The arsN1 gene encodes an N-acetyltransferase that confers resistance to arsinothricin with high selectivity over the related antibiotic phosphinothricin. Here we show that ArsN1 acetylates both AST and PPT but with higher affinity for AST, indicating that ArsN1 is an AST-selective N-acetyltransferase. The overall conformation is a three-layer α/β sandwich fold, a typical GCN5-related N-acetyltransferase fold. PpArsN1 forms an asymmetric homodimer in solution, as shown by the extensive interactions of the subunits and size-exclusion chromatography, similar to related N-acetyltransferases.

The AST-bound PpArsN structure shows that the L-enantiomer is the substrate of the N-acetyltransferase, which supports our assumption that L-AST is the active form of the antibiotic. PpArsN1 has two L-AST-binding sites, which are asymmetrically formed by amino acid residues from both Chains A and B. Both binding sites are composed of seven residues: four residues from Chain A (Ile31a, Phe33a, Ala124a and Val158a) (green) and three residues from Chain B (Arg75b, Ala76b and Arg77b) (teal). A similar water molecule bridge was also observed between AST and Asp85 in AST-bound PpArsN1. We propose that the small difference in the As–O and P–O bond lengths allows L-AST to bind more tightly to PpArsN1 than L-PPT. In L-AST-bound PpArsN1, the bond lengths of As–CG, As–CE, As–OEA, As–OEB are 2.0, 1.9, 1.9 and 2.0 Å, respectively. The volume of the L-AST tetrahedron is 3.00 Å3, compared with 1.86 Å3 for L-PPT. We predict that this substantial difference in substrate volume affects hydrogen bonding, hydrophobic and van der Waal contacts between the tetrahedral substrates and enzyme that accounts in part for the 100-fold higher affinity of ArsN1 for L-AST compared with L-PPT.

>[6x]MHSGIDIRVARPEDAEEIQIIYAPIVLNTAISFEEAVPSVEQMRERISTTLQTYPYLVAVREGRVVGYAYASQHRARAAYRWAVDVTVYVAEGQRRSGIARQLYDVLLPVLKRLGYRSAYAGIALPNEGSVGLHERLGFQHIGTFPQVGFKLDAWHDVGYWRFDFGDEGLHPEAPLGFLSQIPLGPEQKLISEEDLNSAVDHHHHHH>MGGSHHHHHHGMASWSHPQFEKGGHHHHHHGGSGENLYFQGGSGPKFNETADKYLKSGSAEAELIILQYIQQDRVSEDDEEWVYNLLEKANNPYIKLNALLWLSAKRKYLTQLSKLWGISENELKSLSQQQPKIGLFPAVDSRKNAFLAKVFVYKLKSEEPIALAILGDKIENFSYLAQLGKQNCLIGFNKNIQGNSWQLAVLATLLVKDEKIISKIAYSGIVLPSGEIITAEEIEYKKRCCQNLVHRIKKIEQLDAWLNTETIPLPVIQYQGEENELKRWQKAMEQKVQEKFSWFSYELLEDFYGITNSDLAIFGNGILPFEANAWQKLLQEQVKDKFKLLEDKVMPKKVLWFYAGQISTLQLGIGALFGFKRAVSILQMEFSNTTYHEVFILYGKENARQLKNVSVKKEDYQYIQSELLINEPHKNELGFIIYLGSHNPIGEAKAYCQKQLQINNFLIIQARENQGVMETSQNWLPYLQEINSALNTARQEYHWERIHLFQTA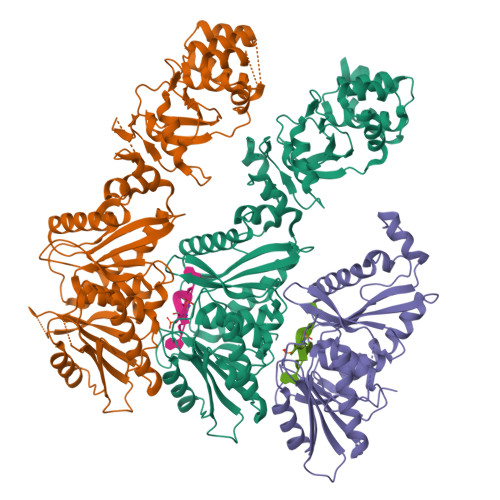PTALCMALGIAVGHFLPVDVYHYQFNAEEPKYRCVFSLDKMLNL[3x]>[2x]MKLFYKPGACSLASHITLRESGKDFTLVSVDLMKKRLENGDDYFAVNPKGQVPALLLDDGTLLTEGVAIMQYLADSVPDRQLLAPVNSIS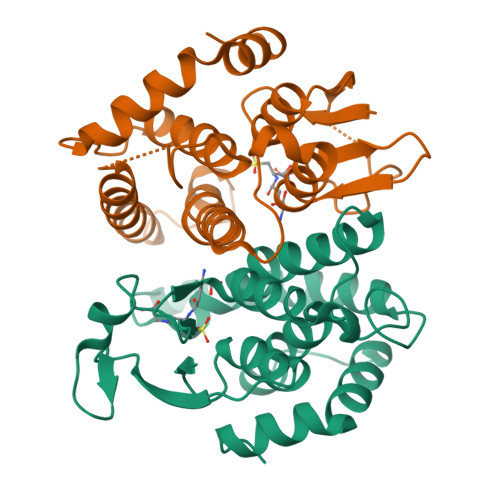RYKTIEWLNYIATELHKGFTPLFRPDTPEEYKPTVRAQLEKKLQYVNEALKDEHWICGQRFTIADAYLFTVLRWAYAVKLNLEGLEHIAAFMQRMAERPEVQDALSAEGLK methyl 3-O-[3-(benzyloxy)-3-oxopropanoyl]-beta-D-galactopyranoside 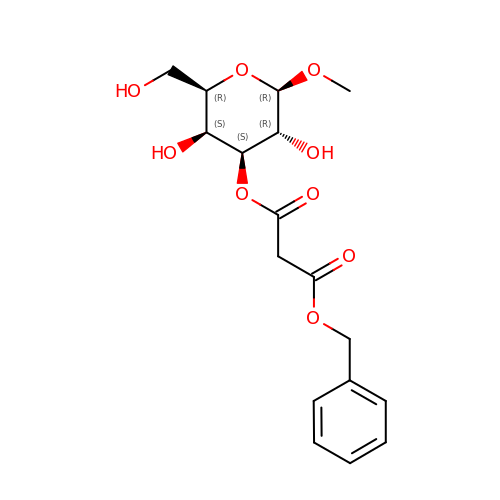| C17 H22 O9 | NMJLHFMLSWSVNI-GNXUOLQESA-N>SNAQFRHLPMPFHWKQEELKFKTGLRRLQHRVGEIHLLREALQKGAEAGQVSLHSLIETPANGTGPSEALAMLLQETTGELEAAKALVLKRIQIWKRQQQLAGNGAPFEESLAPLQERCESLVDIYSQLQQEVGAAGGELEPKTRASLTGRLDEVLRTLVTSCFLVEKQPPQVLKTQTKFQAGVRFLLGLRFLGAPAKPPLVRADMVTEKQARELSVPQGPGAGAESTGEIINNTVPLENSIPGNCCSALFKNLLLKKIKRCERKGTESVTEEKCAVLFSASFTLGPGKLPIQLQALSLPLVVIVHGNQDNNAKATILWDNAFSEMDRVPFVVAERVPWEKMCETLNLKFMAEVGTNRGLLPEHFLFLAQKIFNDNSLSMEAFQHRSVSWSQFNKEILLGRGFTFWQWFDGVLDLTKRCLRSYWSDRLIIGFISKQYVTSLLLNEPDGTFLLRFSDSEIGGITIAHVIRGQDGSPQIENIQPFSAKDLSIRSLGDRIRDLAQLKNLYPKKPKDEAFRSHYKPE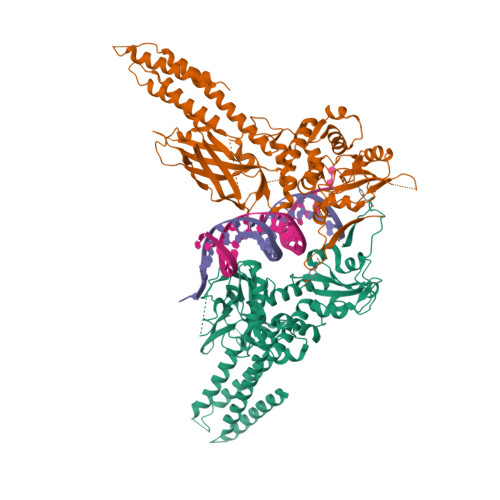QMGKDGRGYVPATIKMTVERDQPLPT[4x]>MKKENQTQEIEERYQALFSN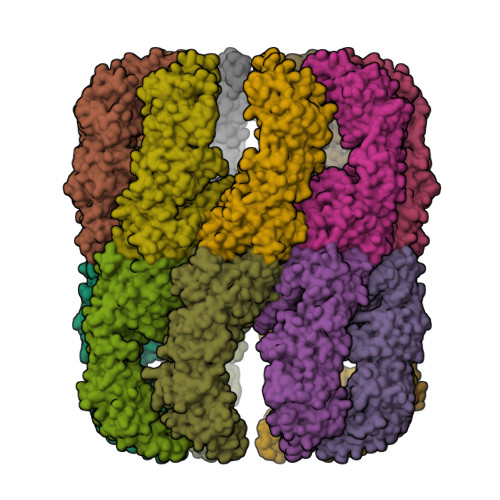AAAVKALTQVVANSLGPKGLDAMLVDRFGEVVVTNDGVTILTLMDAQHPAARMVVNMARAQEREVGDGTTTAAVLAGALVSEGVNQILKGVPVSKVLAGMNRALNHALFLIRKNAIKVGSITDDRLLAAAKIAGRGDERVAAILRDAAAMLEDKLQDPGFKLADLVLAKVGADTTLIPGVVINKSPLWEEGSQKLQEVRLLVLDDGLYPEEVEEEALASEAGFEQYLKNQKIFQENLKKLKELGVKLILLTRGISDIAEEFCYENEIMVITRITQKELKRVLEFTGARAAKRTSLNKPVEELQKMLGYARTCFYDSRLDFTIIEGGAGKATATVLIGAATDEVVDEQERIAKDAAGSFAAAYRSGVLPGGGAFFLYLSREVESLKNRLPGMESYGVMAFSEALKVPFRVMAENAGFNGLEKLGDLMTLQVQKNNYALGLDFETGEFIDMIAGGVVDPAEVVYQAVKNASEVAISLLKINTIIKMKDYEVLKEGEQEDGGKR[4x]> GPLGSAVSLVQAQTNARAIAAMKNSIQATNRAVFEVK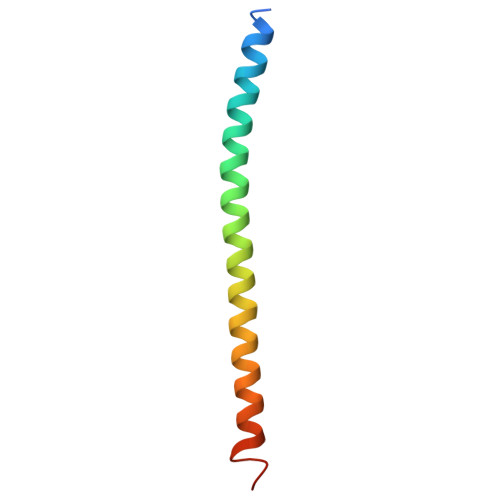EGTQRLAIAVQAIQDHINTIMNTQLN>MFRNHASRITAAAAPWVLRTACRQKSDAKTPVWGHTQLNRLSFLETVPVVPLRVSDESSEDRPTWSLPDIENVAITHKKPNGLVDTLAYRSVRTCRW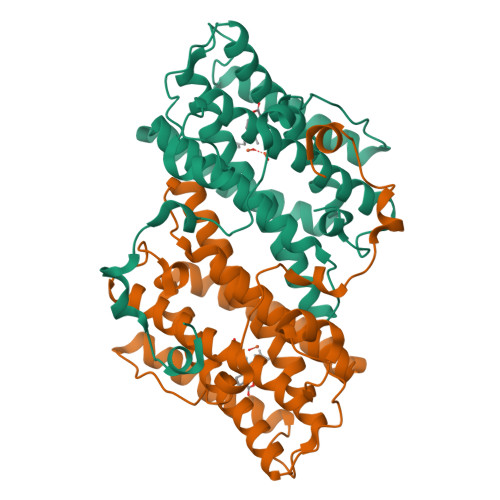LFDTFSLYRFGSITESKVISRCLFLETVAGVPGMVGGMLRHLSSLRYMTRDKGWINTLLVEAENERMHLMTFIELRQPGLPLRVSIIITQAIMYLFLLVAYVISPRFVHRFVGYLEEEAVITYTGVMRAIDEGRLRPTKNDVPEVARVYWNLSKNATFRDLINVIRADEAEHRVVNHTFADMHEKRLQNSVNPFVVLKKNPEEMYSNQPSGKTRTDFGSEGAKTASNVNKHV[4x]> GAMDPEFSAQLGAMQHLKDQLEQRTRMIEAN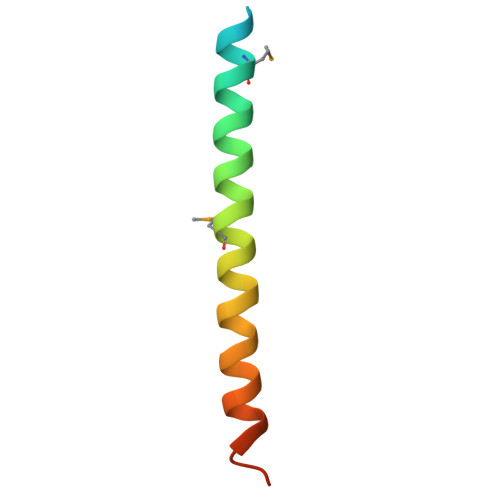IHRQQEELRKIQEQLQMVHG>[4x]TSACENFLLPADQDGIQRQVTIFRYGQENSAPKAYLQAGLHADEFPGMLALKYLRDLLDEAARRNR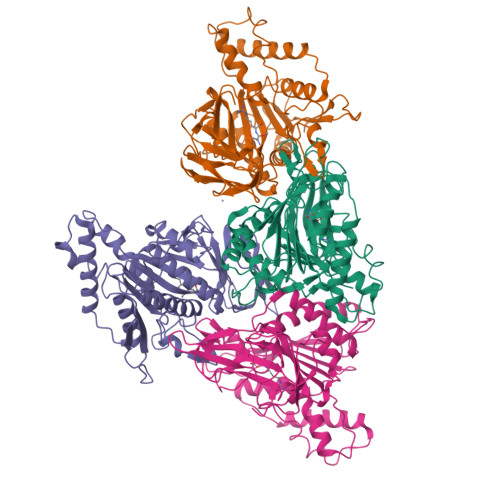IKGEIVIIPQANPIGLSQWKDGFLLGRFDHQTGTNFNRDYPDLCQLTVEKLDGQLTENAEHNIDVIRKTMRSALSELKPEQAVDVLRHKLISESCDADLVLDLHADNQAQCHMYTLTPLWPAMHDVAAEIDARAVLLAEESGGHPFDEACSAPWMNLSRAFPDYPIPLACQSATFALGSNDEVDLRLAQDQAEALFRILIRRGFIEDVHVGELPQLACEGTLLEAMQQLKAPCQGLIVYHNRLGDFVRSGDKVVSIVDPIGETVDILAHTDGVLFARHSQTYAYPNKVIGKIAGKEPLPERKGF>[2x]SLSFRMSPTQKETRL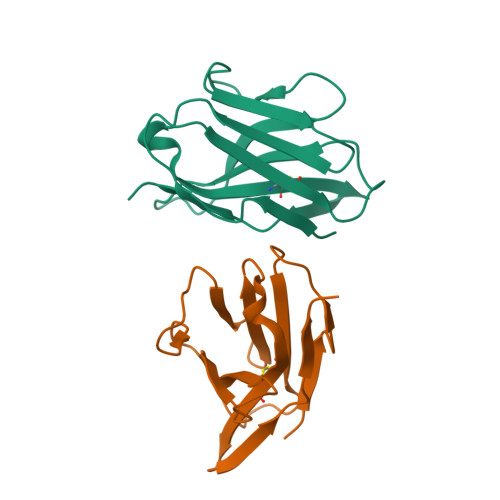GEKVELQCELLQSGMATGCSWLRHIPGDDPRPTFLMYLSAQRVKLAEGLDPRHISGAKVSGTKFQLTLSSFLQEDQGYYFCSVVSNSILYFSNFVPVFLP> KELLDSDGDILRNGGTYYILPALRGKGGGLELAKTGDETCPLNVVQARSETKRGRPAIIWTPPRI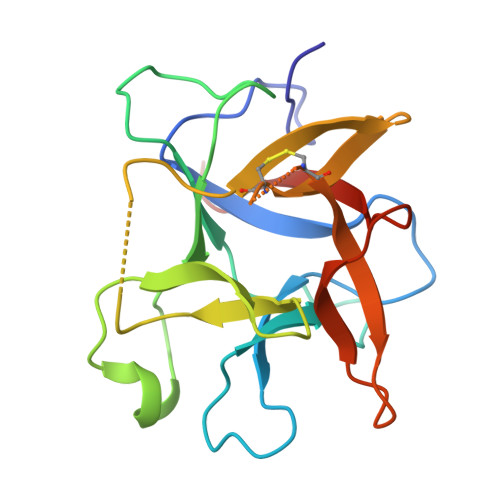AILTPAFYLNIEFQTRDLPACLEEYSRLPWKVEGESQEVKIAPKEEEQHLFGSFKIKPYRDDYKLVYCEGNSDDDSCKDLGISIDDENNRLLVVKDGDPLAVRFVKAHRRG>[4x]TQFDKQYNSIIKDIINNGISDEEFDV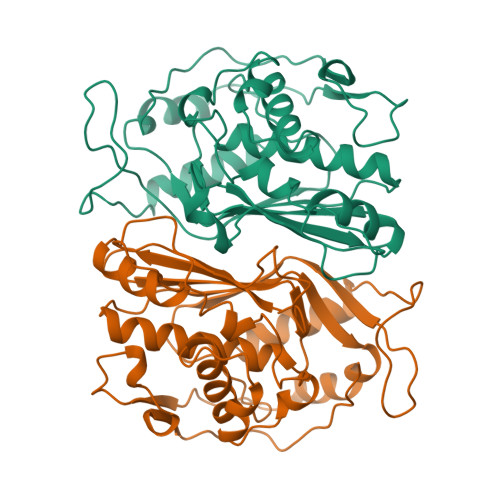RTKWDSDGTPAHTLSVISKQMRFDNSEVPILTTKKVAWKTAIKELLWIWQLKSNDVNDLNMMGVHIWDQWKQEDGTIGHAYGFQLGKKNRSLNGEKVDQVDYLLHQLKNNPSSRRHITMLWNPDELDAMALTPCVYETQWYVKHGKLHLEVRARSNDMALGNPFNVFQYNVLQRMIAQVTGYELGEYIFNIGDCHVYTRHIDNLKIQMEREQFEAPELWINPEVKDFYDFTIDDFKLINYKHGDKLLFEVAV>[6x]LNSVGQGEFGGAPFKRFLRGTRIVSGGKLKRMTREKAKQVTVAGVPMPRDAEPRHLLVNG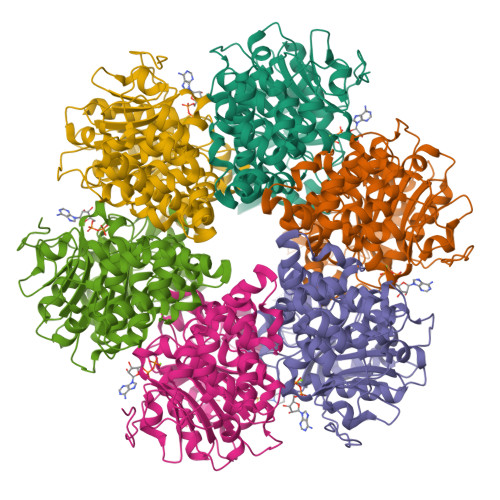ATGTGKSVLLRELAYTGLLRGDRMVIVDPNGDMLSKFGRDKDIILNPYDQRTKGWSFFNEIRNDYDWQRYALSVVPRGKTDEAEEWASYGRLLLRETAKKLALIGTPSMRELFHWTTIATFDDLRGFLEGTLAESLFAGSNEASKALTSARFVLSDKLPEHVTMPDGDFSIRSWLEDPNGGNLFITWREDMGPALRPLISAWVDVVCTSILSLPEEPKRRLWLFIDELASLEKLASLADALTKGRKAGLRVVAGLQSTSQLDDVYGVKEAQTLRASFRSLVVLGGSRTDPKTNEDMSLSLGEHEVERDRYSKNTGKHHSTGRALERVRERVVMPAEIANLPDLTAYVGFAGNRPIAKVPLEIKQFANRQPAFVEGTI>[2x]MVVTCPKCGAKNRLG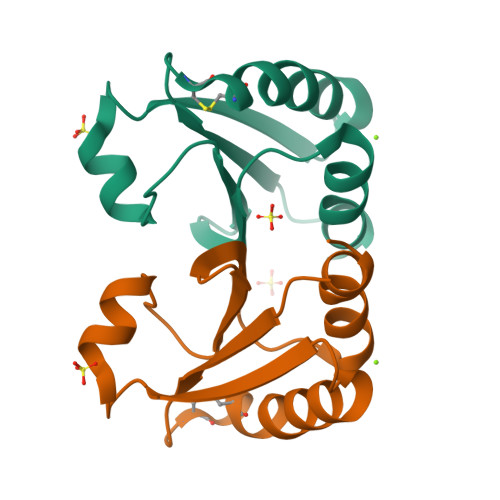TPPPGQVPVCGACKTPLPWVVEADEKGFAQEVAGAPLTLVDFFAPWCGPCRLVSPILEELARDHAGRLKVVKVNVDEHPGLAARYGVRSVPTLVLFRRGAPVATWVGASPRRVLEERLRPYLEGR(4S)-4-methyl-2,5,7-trioxoheptanoic acid | C8 H10 O5 | 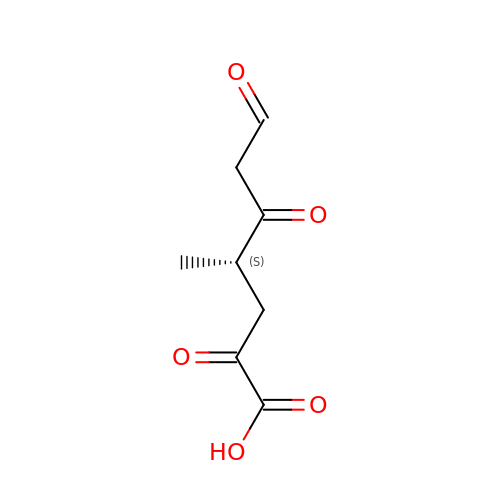JDEHLHSRIXMJEO-YFKPBYRVSA-N>MDKQHFKLWYFQFRGRAEPIRLLLTCAGVKFEDYQFTMDQWP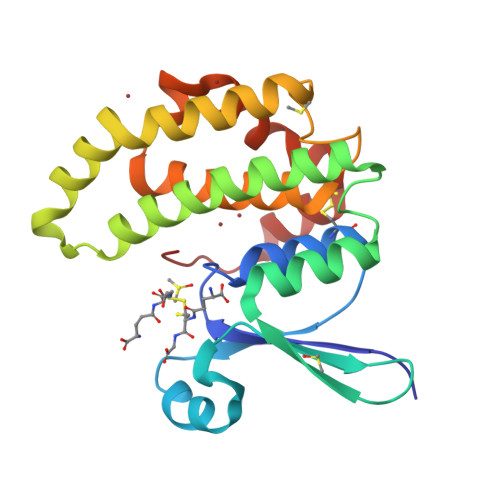TIKPTLPGGRVPLLDVTGPDGKLRRYQESMAIARLLARQFKMMGETDEEYYLIERIIGECEDLYREVYTIFRTPQGEKEAKIKEFKENNGPTLLKLVSESLESSGGKHVAGNRITLGDLFLFTTLTHVMETVPGFLEQKFPKLHEFHKSLPTSCSRLSEYLKKRAKTPF[2x]> EDDLYRQSLEIISRYLREQATGSKDSKPLGEAGAAGRRALETLRRVGDGVQRNHETAFQGMLRKLDIKNEDDVKSLSRVMIHVFSDGVTNWGRIVTLISFGAFVAKHLKTINQESCIEPLAESITDVLVRTKRDWL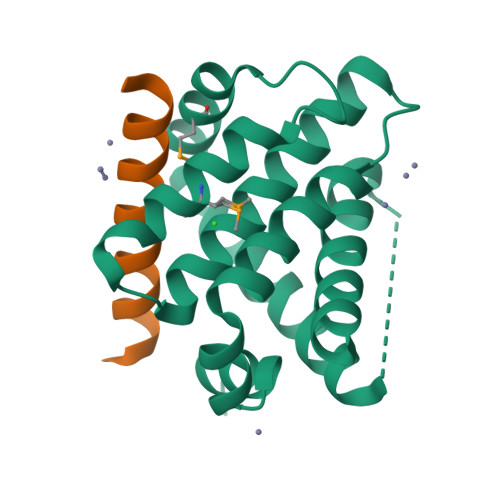VKQRGWDGFVEFFHVEDLEGG;> DMRPEIWIAQELRRIGDEFNAYYARR>[5x]LSPSFGSTWSTGTTNAVE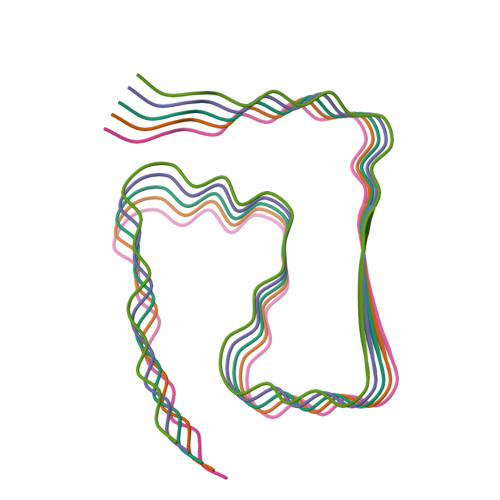DSFFQGITPVNGTMLFQNFPHHVNPVFGGTF>[6x]MAGFWVGTAPLVAAGRRGRWPPQQLMLSAALRTLKHVLYYSRQCLMVSRNLGSVGYDPNEKTFDKILVANRGEIACRVIRTCKKMGIKTVAIHSDVDASSVHVKMADEAVCVGPAPTSKSYLNMDAIMEAIKKTRAQAVHPGYGFLSENKEFARCLAAEDVVFIGPDTHAIQAMGDKIESKLLAKKAEVNTIPGFDGVVKDAEEAVRIAREIGYPVMIKASAGGGGKGMRIAWDDEETRDGFRLSSQEAASSFGDDRLLIEKFIDNPRHIEIQVLGDKHGNALWLNERECSIQRRNQKVVEEAPSIFLDAETRRAMGEQAVALARAVKYSSAGTVEFLVDSKKNF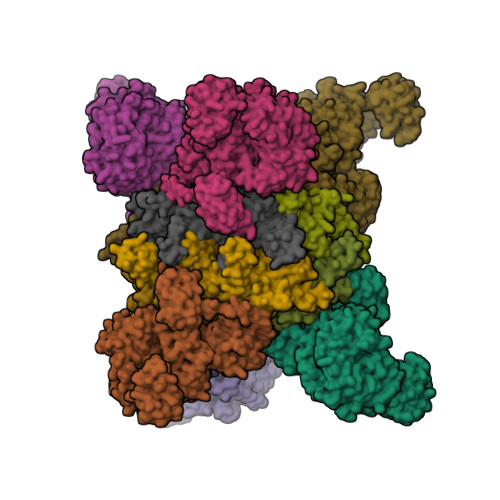YFLEMNTRLQVEHPVTECITGLDLVQEMIRVAKGYPLRHKQADIRINGWAVECRVYAEDPYKSFGLPSIGRLSQYQEPLHLPGVRVDSGIQPGSDISIYYDPMISKLITYGSDRTEALKRMADALDNYVIRGVTHNIALLREVIINSRFVKGDISTKFLSDVYPDGFKGHMLTKSEKNQLLAIASSLFVAFQLRAQHFQENSRMPVIKPDIANWELSVKLHDKVHTVVASNNGSVFSVEVDGSKLNVTSTWNLASPLLSVSVDGTQRTVQCLSREAGGNMSIQFLGTVYKVNILTRLAAELNKFMLEKVTEDTSSVLRSPMPGVVVAVSVKPGDAVAEGQEICVIEAMKMQNSMTAGKTGTVKSVHCQAGDTVGEGDLLVELE;>MAAALRVAAVGARLSVLASGLRAAVRSLCSQATSVNERIENKRRTALLGGGQRRIDAQHKRGKLTARERISLLLDPGSFVESDMFVEHRCADFGMAADKNKFPGDSVVTGRGRINGRLVYVFSQDFTVFGGSLSGAHAQKICKIMDQAITVGAPVIGLNDSGGARIQEGVESLAGYADIFLRNVTASGVIPQISLIMGPCAGGAVYSPALTDFTFMVKDTSYLFITGPDVVKSVTNEDVTQEELGGAKTHTTMSGVAHRAFENDVDALCNLRDFFNYLPLSSQDPAPVRECHDPSDRLVPELDTIVPLESTKAYNMVDIIHSVVDEREFFEIMPNYAKNIIVGFARMNGRTVGIVGNQPKVASGCLDINSSVKGARFVRFCDAFNIPLITFVDVPGFLPGTAQEYGGIIRHGAKLLYAFAEATVPKVTVITRKAYGGAYDVMSSKHLCGDTNYAWPTAEIAVMGAKGAVEIIFKGHENVEAAQAEYIEKFANPFPAAVRGFVDDIIQPSSTRARICCDLDVLASKKVQRPWRKHANIPL[6x]> EEVEMAKRRIDEINKELNQVMEQLGDARIDRQESSRQQRKAEIMESIKRLYPGSVYGRLIDLCQPTQKKYQIAVTKVLGKNMDAIIVDSEKTGRDCIQYIKEQRGEPETFLPLDYLEVKPTDEKLRELKGAKLVIDVIRYEPPHIKKALQYACGNALVCDNV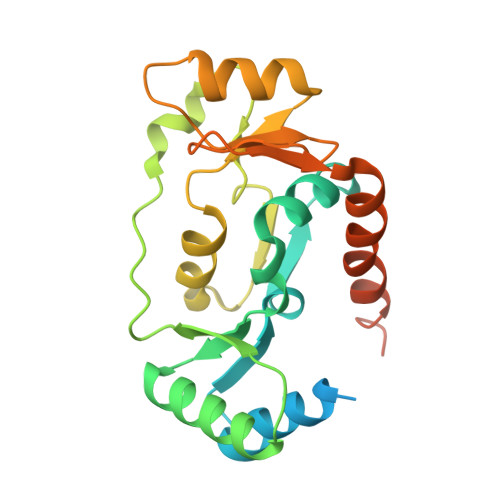EDARRIAFGGHQRHKTVALDGTLFQKSGVISGGASDLKAKARRWDEKAVDKLKEKKGRLTEELLEHHHHHH>GSMAWFFGKIPRAKAEEMLSKQRHDGAFLIRESESAPGDFSLSVKFGNDVQHFKVLRDGAGKYFLWVVKFNSLNELVDYHRSTSVSR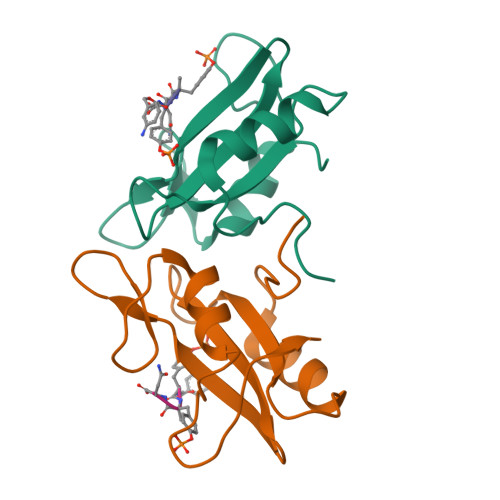NQQIFLRDI[2x]> MPFVNKQFNYKDPVNGVDIAYIKIPNAGQMQPVKAFKIHNKIWVIPERDTFTNPEEGDLNPPPEAKQVPVSYYDSTYLSTDNEKDNYLKGVTKLFERIYSTDLGRMLLTSIVRGIPFWGGSTIDTELKVIDTNCINVIQPDGSYRSEELNLVIIGPSADIIQFECKSFGHEVLNLTRNGYGSTQYIRFSPDFTFGFEESLEVDTNPLLGAGKFATDPAVTLAHELIHAGHRLYGIAINPNRVFKVNTNAYYEMSGLEVSFEELRTFGGHDAKFIDSLQENEFRLYYYNKFKDIASTLNKAKSIVGTTASLQYMKNVFKEKYLLSEDTSGKFSVDKLKFDKLYKMLTEIYTEDNFVKFFKVLNRKTYLNFDKAVFKINIVPKVNYTIYDGFNLRNTNLAANFNGQNTEINNMNFTKLKNFTGLFEHHHHHH;> QRATKMX

Seven antigenically distinct botulinum neurotoxins are produced by the bacterium Clostridium botulinum and they share considerable sequence homology, and structural and functional similarity. They are produced as inactive single chains of molecular mass 150 kDa and released as active dichains, a heavy chain (HC, 100 kDa) and a light chain (LC, 50 kDa) held together by an interchain disulfide bond. HC comprising two distinct domains is responsible for binding to neuronal cells and translocation into cytosol. LC is the catalytic domain cleaving one of the three proteins forming the SNARE complex (Soluble N-ethylmaleimide-sensitive fusion protein attachment protein receptors) required for docking and fusion of vesicles containing neurotransmitters to target cells. Catalytic domains of BoNTs are zinc proteases and cleave SNARE proteins with stringent substrate specificity though they share significant sequence similarity. BoNT/A and BoNT/E cleave the synaptosomal-associated 25 kDa protein (SNAP-25) while BoNT/B, /D, /F, and /G cleave the vesicle-associated membrane protein (VAMP).

Here we present for the first time the structure of the substrate peptide, QRATKM containing the scissile peptide bond, bound to the active enzyme. The crystal structure has been determined to 1.5Å resolution. The final refined model contains 423 protease residues, 6 substrate residues, one sulfate and one zinc ions and 375 waters. The electron density in the residual map (Fo-Fc) was well defined for the hexapeptide and QRATKM could be modeled unambiguously except for the side chains of K and M. It appears that K could take two rotamer positions. This is the first time an uncleavable substrate bound structure of an active botulinum neurotoxin has been reported and it has helped in unequivocally defining S1 to S5′ sites. Most notably, the amino nitrogen and carbonyl oxygen of P1 residue (Gln197) chelate the zinc ion. The amino nitrogen has replaced the nucleophilic water as was shown earlier. The side chain of P1-Q197 is exposed to the solvent region but makes a hydrogen bond with Glu164 OE1. While SN/A1 was cleavable by BoNT/A, SN/A2 was not, suggesting that the N terminal DEAN is required for cleavage. This probably explains why QRATKM which lacks DEAN was not cleaved in our case even though we used up to 1∶30 ratio of Balc424 to peptide. However, the major reason for the peptide not being cleaved is the amino group chelating zinc.[(2S)-5-oxo-2,5-dihydrofuran-2-yl]acetic acid | C6 H6 O4 | 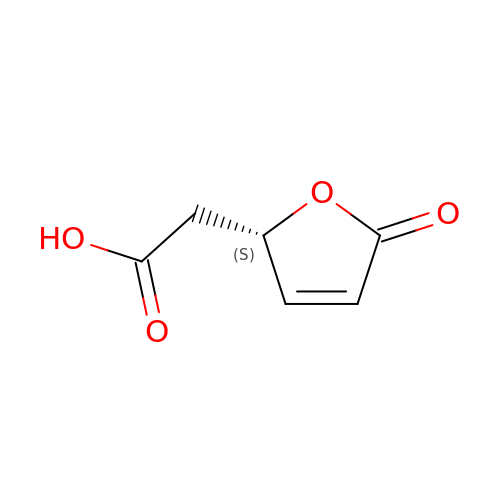HPEKPJGPWNSAAV-SCSAIBSYSA-N> GEEDLCAAFNVICDNVGKDWRRLARQLKVSDTKIDSIEDRYPRNL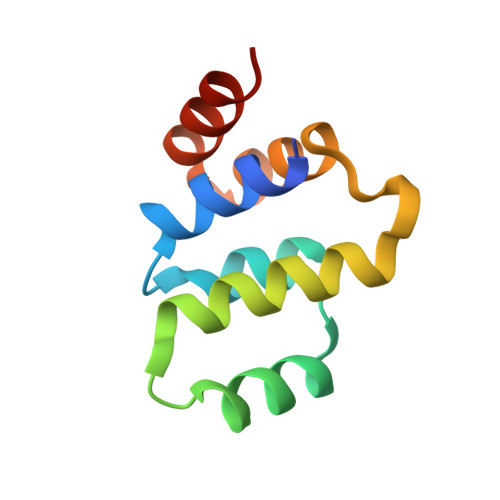TERVRESLRIWKNTEKENATVAHLVGALRSCQMNLVADLVQEVQQAR> MKKFRKHKRISNCISILLILYLTLGGLLPNNIYAQDLQSYSEKVCNTTYKAPIERPEDFLKDKEKAKEWERKEAERIEQKLERSEKEALESYKKDSVEISKYSQTRNYFYDYQIEANSREKEYKELRNAISK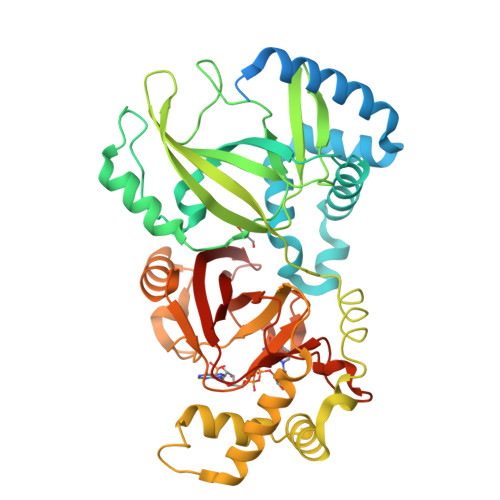NKIDKPMYVYYFESPEKFAFNKVIRTENQNEISLEKFNEFKETIQNKLFKQDGFKDISLWEPGKGDEKPTPLLMHLKLPRNTGMLPYTNTNNVSTLIEQGYSIKIDKIVRIVIDGKHYIKAEASVVSSLDFKDDVSKGDSWGKANYNDWSNKLTPNELADVNDYMRGGYTAINNYLISNGPVNNPNPELDSKITNIENALKREPIPTNLTVYRRSGPQEFGLTLTSPEYDFNKLENIDAFKSKWEGQALSYPNFISTSIGSVNMSAFAKRKIVLRITIPKGSPGAYLSAIPGYAGEYEVLLNHGSKFKINKIDSYKDGTITKLIVDATLIP> SSVALIVGVTGIIGNSLAEILPLADTPGGPWKVYGVARRTRPAWHE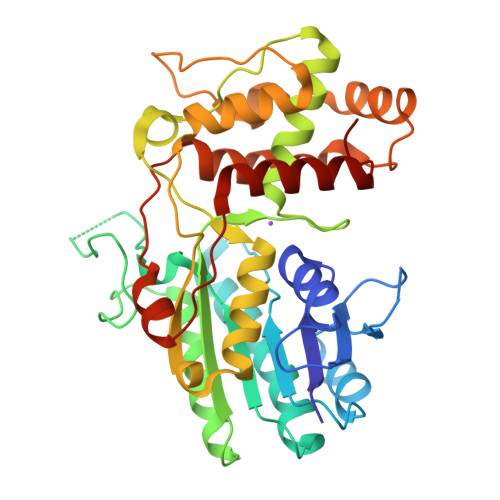DNPINYVQCDISDPDDSQAKLSPLTDVTHVFYVTWANRSTEQENCEANSKMFRNVLDAVIPNCPNLKHISLQTGRKHYMGPFESYGKIESHDPPYTEDLPRLKYMNFYYDLEDIMLEEVEKKEGLTWSVHRPGNIFGFSPYSMMNLVGTLCVYAAICKHEGKVLRFTGCKAAWDGYSDCSDADLIAEHHIWAAVDPYAKNEAFNVSNGDVFKWKHFWKVLAEQFGVECGEYEEGVDLKLQDLMKGKEPVWEEIVRENGLTPTKLKDVGIWWFGDVILGNECFLDSMNKSKEHGFLGFRNSKNAFISWIDKAKAYKIVP We report biochemical properties and crystal structures of the LD-carboxypeptidases LdcB from Streptococcus pneumoniae, Bacillus anthracis, and Bacillus subtilis. The enzymes are active against bacterial cell wall tetrapeptides and adopt a zinc-carboxypeptidase fold characteristic of the LAS superfamily. LD-carboxypeptidases subsequently hydrolyze the L-Lys[A2pm]—D-Ala bond to release the tripeptide. The LdcB enzymes are single domain proteins comprising two subdomains separated by a V-shaped cleft.

The crystal structures of SpLdcB and Bacillus anthracis LdcB (BaLdcB) were solved by single wavelength anomalous dispersion (SAD); BsLdcB was solved by molecular replacement. In SpLdcB, the liganding residues are His153, Asp160, and His207; the equivalents in BsLdcB/BaLdcB are His185/His160, Asp192/Asp167, and His244/His219. The active site of SpLdcB contains unattributed residual electron density that occupies the position of the fourth ligand in the tetrahedral coordination sphere of the zinc. To use the nomenclature common to proteases, the unattributed electron density extends as far as the S1′ subsite, the location ordinarily occupied by the scissile amino acid. The electron density in the S1′ subsite is of a size, shape, and location corresponding to that of alanine. The ligand is stabilized in this position by van der Waals’ contacts between the alanyl methyl group and the phenolic side chains of Tyr191 and Tyr201 and by hydrogen bonds to the side chains of Glu204 and the main chain amide nitrogen of Tyr144. Despite the high resolution of the SpLdcB diffraction data, it was not possible to discriminate between either alanyl stereoisomer, both of which are present in the crystallization conditions. We have modeled D-Ala because it is the enzymatic product of these enzymes. However, residual electron density adjacent to the zinc ion could not be modeled satisfactorily with any ligand arising from the enzymatic activity, the crystallization media, or purification media; consequently, the remaining electron density has been left unmodeled. First and foremost, substrates are occluded in the empty form of the enzyme by a loop between residues Gly163 and Glu171, which blocks access to the active site.

> GSHMEVVNKGDYYSIQGKYDEIIVANKHYPLSKDYNPGENPTAKAELVKLIKAMQEAGFPISDHYSGFRSYETQTKLYQDYVNQDGKEAADRYSARPGYSEHQTGLAFDVIGTDGDLVTEEKAAQWLLDHAADYGFVVRYLKGKEKETGYMAEEWHLRYVGKEAKEIAESGLSLEEYYGFEGGDYVD>[2x]MGS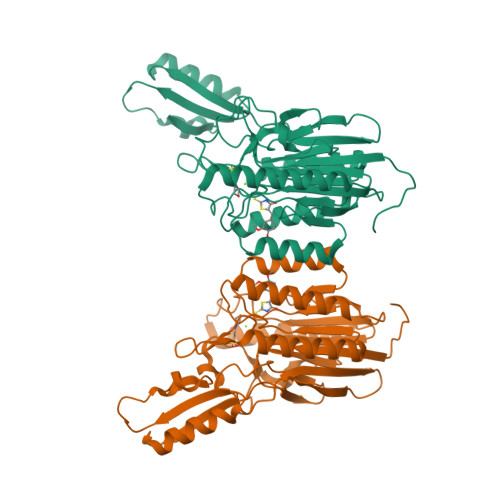DKIHHHHHHVINLKELKILHTSDWHLGVTSWTSSRPVDRREELKKALDKVVEEAEKREVDLILLTGDLLHSRNNPSVVALHDLLDYLKRMMRTAPVVVLPGNHDWKGLKLFGNFVTSISSDITFVMSFEPVDVEAKRGQKVRILPFPYPDESEALRKNEGDFRFFLESRLNKLYEEALKKEDFAIFMGHFTVEGLAGYAGIEQGREIIINRALIPSVVDYAALGHIHSFREIQKQPLTIYPGSLIRIDFGEEADEKGAVFVELKRGEPPRYERIDASPLPLKTLYYKKIDTSALKSIRDFCRNFPGYVRVVYEEDSGILPDLMGEIDNLVKIE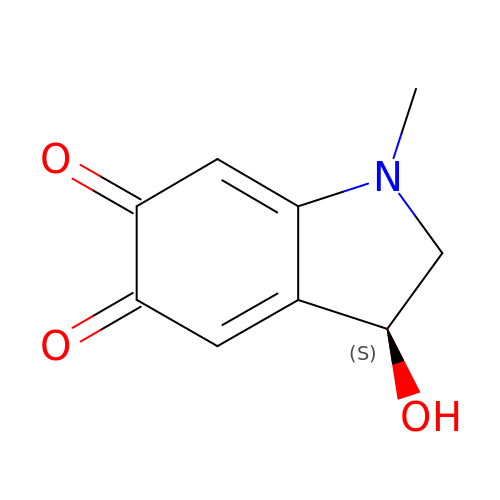(3S)-3-hydroxy-1-methyl-2,3-dihydro-1H-indole-5,6-dione | C9 H9 N O3 | RPHLQSHHTJORHI-SECBINFHSA-N> MGSSHHHHHHSSGLVPRGSLKGNIRVFCRVRPVLPGEPTPPPGLLLFPSGPGGPSDPPTRLSLSRSDERRGTLSGAPAPPPRHDFSFDRVFP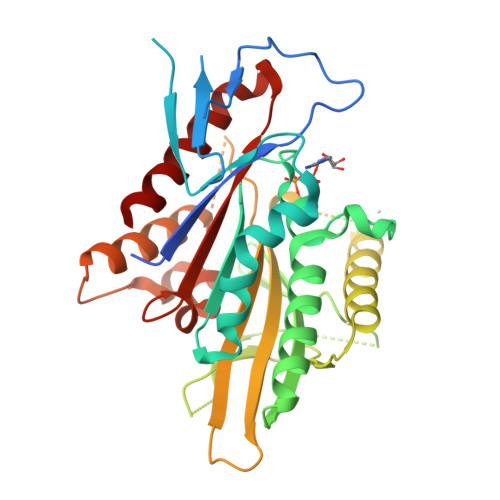PGSGQDEVFEEIAMLVQSALDGYPVCIFAYGQTGSGKTFTMEGGPGGDPQLEGLIPRALRHLFSVAQELSGQGWTYSFVASYVEIYNETVRDLLATGTRKGQGGECEIRRAGPGSEELTVTNARYVPVSCEKEVDALLHLARQNRAVARTAQNERSSRSHSVFQLQISGEHSSRGLQCGAPLSLVDLAGSERLDPGLALGPGERERLRETQAINSSLSTLGLVIMALSNKESHVPYRNSKLTYLLQNSLGGSAKMLMFVNISPLEENVSESLNSLRFASKVNQC>[4x]MAQDMSPRQSAEAFGVPAVSSSWVNQDGSTMTLVFGAGNSVSGF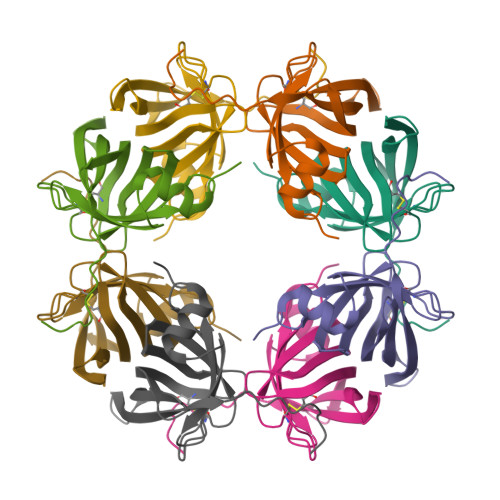YVNNAPGFGCQGTPYPLVGLTWGNFIGFTVAWDNATANCNSVTSWTGFAEAAGSDVTIVTDWNLAYQGSSSGEIQQGSDTFTLVNKAMKETPKM>MFNNEPLEQIDKELHDILADEEKRQRETINLIASENLTNGAVRECLGNRVSNKYSEGYPKKRYYGGNDFIDKIEELCQKRALEAFNVSDEEWGVNVQPLSGSAANVQALYALVGVKGKIMGMHLCSGGHLTHGFFDEKKKVSITSDMFESKLYKCNSQGYVDLDAVREMALSFKPKVIICGYTSYPRDIDYQQFRQICDEVNAYLFADISHISSFVACNILNNPFLHADVVTTTTHKILRGPRSALIFFNKKRNPGIEQKINSAVFPSFQGGPHNNKIAAVACQLKEVHSPAFKEYTQQVLLNSKALAKALISKQIDLVTNGTDNHLIVVDLRKFSITGSKLQETCNAINVSLNKNTIPSDVDCVSPSGVRIGTPAMTTRGAKEKDMEFIADVLARAIKITVDLQEQYGKKLVDFKKGLPGNAQLQQLKQEVVTWAGALPFP[3x]

SHMT is a pyridoxal-5′-phosphate (PLP)-dependent enzyme that catalyzes the interconversion of l-serine (l-Ser) and tetrahydro­folate (THF) to glycine (Gly) and methylene tetrahydrofolate (MTHF). The enzyme provides activated one-carbon units for the synthesis of dTMP, choline and amino acids. Plasmodium serine hydroxymethyltransferase (SHMT) has recently been shown to be vital for parasite growth and development, making it a potential target for antimalarial drug development. The overall structure of PvSHMT was found to be very similar to that of PfSHMT, existing as a twofold symmetric homodimer with two catalytic sites.

The first was a crystal of the binary complex of PvSHMT with l-Ser, which diffracted to 2.5 Å resolution and was obtained in the presence of methotrexate (MTX), although there was no density for MTX in the final map. The structures of the PvSHMT–l-Ser and PvSHMT–d-Ser–5FTHF complexes were used to assess the amino-acid binding pocket. Key interactions with both d-Ser and l-Ser consist of two components: hydrogen bonds from the conserved residues in the PLP pocket (Ser100, Ser102, Thr183, Asp208, His129, His236, Tyr′54 and Gly′272) and the amino-acid pocket (Ser34, His211, Arg371, Glu′56 and Tyr′64). Although the stabilizing interactions are from identical residues, three major differences between d-Ser and l-Ser binding can be observed. Firstly, the salt-bridge interactions between the Arg371 side chain and the carboxyl group of d-Ser are distorted, at distances of 3.0 and 3.2 Å, while two ideal salt bridges at distances of 2.7 and 2.8 Å are observed to l-Ser. The d-Ser side chain is oriented away from N5 of THF and is found in the extended plane of the PLP ring, while the l-Ser side chain is perpendicular to N5. Differences in the accommodation of l-Ser and d-Ser in the PvSHMT active site may account for the broad substrate specificity of SHMT and the lower catalytic efficiency for d-Ser in the THF-dependent catalytic function. Nevertheless, these observations indicate that the overall amino-acid binding site of PvSHMT is sufficiently plastic to accommodate both the d- and l-isomers of the substrate. The crystal structures of complexes of PvSHMT with l-Ser and d-Ser–(6R)-5FTHF revealed that the arrangement of the residues in the amino-acid binding pocket is restricted by the configuration of the bound amino-acid substrate, leading to different catalytic efficiencies towards each substrate isomer.N-{(3S)-1-[5-(propan-2-yl)-1H-pyrazole-3-carbonyl]pyrrolidin-3-yl}cyclopropanecarboxamide | C15 H22 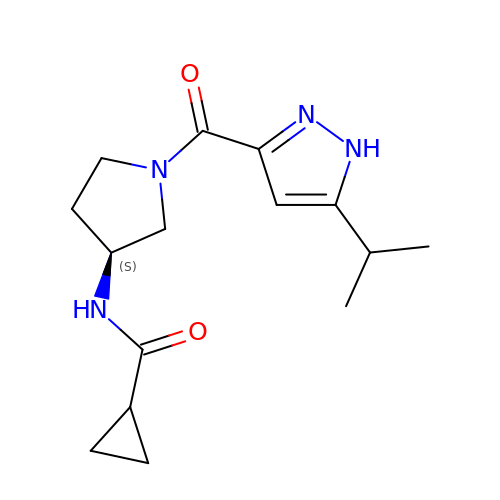N4 O2 | CXEXTVGTDZRKJS-NSHDSACASA-N Among all bacterial pathogens, Legionella pneumophila maintains the largest known set of translocated substrates, delivering over 300 proteins to the host cell via its Type IVB, Icm/Dot translocation system. In at least nine instances, this regulation is direct—a hallmark of an emerging class of proteins called metaeffectors, or “effectors of effectors”. Through detailed structural and functional analysis, we show that metaeffector activity derives from a diverse range of mechanisms, shapes evolution, and can be used to reveal important aspects of each cognate effector's function. After release into the host cell, translocated bacterial substrates (effectors) regulate one another through several different functional interactions: indirectly, through counteracting modification of a shared host target, or directly through either steric complex formation or direct modification of one effector by another.

In addition to its inhibitory effects on MavQ, SidP synergizes with another effector, Lem14 (Lpg1851), to cause a severe growth defect when co‐expressed in our yeast screen. Strikingly, neither protein confers a measurable growth defect on its own. To explore this further, we solved the crystal structure of Lem14, revealing a small, alpha‐helical protein that forms an anti‐parallel dimer and is structurally similar to another effector, LpiR1, whose molecular function remains elusive (Beyrakhova et al, 2016). A citric acid molecule was found inside a positively charged pocket at the ends of α1–4. Lem14 has a positively charged pocket that is required for SidP‐Lem14 synergy in yeast, as mutants that reverse the charge (inset) alleviate the SidP‐Lem14 yeast growth inhibition. The synergistic effect of SidP and Lem14 is dependent on the SidP phosphatase activity and Lem14's charged pocket. Co‐overexpression of wild‐type SidP and Lem14 caused a sicker than expected growth phenotype in yeast, but any SidP or Lem14 mutant alleviated this effect. While revealing the full mechanistic basis of SidP‐Lem14 synergy remained outside of the scope of this current study, the uniqueness of this pair and its linkage to our earlier work warranted at least some investigation. In contrast to the SidP‐MavQ interaction described above, the synergistic interaction between SidP and Lem14 does not appear to involve a physical interaction as tested by the Y2H assay and LUMIER (Table EV5). Providing further support to an indirect synergistic interaction, we observe clear cross‐species synergy between L. pneumophila Lem14 and SidP from L. dumoffii in our screen. Indeed, together with our suppression data, the observation of SidP‐Lem14 synergy makes SidP a remarkable hub of effector activity within the eukaryotic cell, likely linking SidP/MavQ host lipid modulation with the as‐of‐yet undiscovered function of Lem14.

> GMSFELVAYEKLKGSIRESIITLIKSHNEKAKIIEDKLEYSVKEVSRERQPQVLVLLKTIELLDNSSKEPEDKARVLNALAYYIRDQIAATYKYTSPDNSDFYKSLTISLDLNKDNNPNREDLADMYSALEKFLRSHVYKNSDPRKGYLDKQPFAIKHYSVVDDILELSDRVHKLRHEIIIAARDLHLLQ2',5'-GpAp 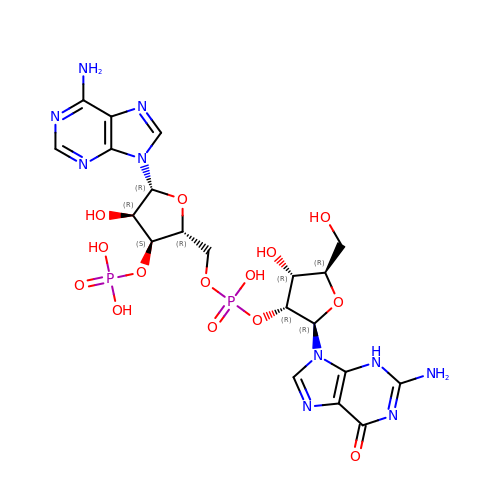| C20 H26 N10 O14 P2 | OVXKSNAROFCXFB-INFSMZHSSA-N> MLRRALLCLAVAALVRADAPEEEDHVLVLRKSNFAEALAAHKYLLVEFYAPWCGHCKALAPEYAKAAGKLKAEGSEIRLAKVDATEESDLAQQYGVRGYPTIKFFRNGDTASPKEYTAGREADDIVNWLKKRTGPAATTLPDGAAAESLVESSEVAVIGFFKDVESDSAKQFLQAAEAIDDIPFGITSNSDVFSKYQLDKDGVVLFKKFDEGRNNFEGEVTKENLLDFIKHNQLPLVIEFTEQTAPKIFGGEIKTHILLFLPKSVSDYDGKLSNFKTAAESFKGKILFIFIDSDHTDNQRILEFFGLKKEECPAVRLITLEEEMTKYKPESEELTAERITEFCHRFLEGKIKPHLMSQELPEDWDKQPVKVLVGKNFEDVAFDEKKNVFVEFYAPWCGHCKQLAPIWDKLGETYKDHENIVIAKMDSTANEVEAVKVHSFPTLKFFPASADRTVIDYNGERTLDGFKKFLESGGQDGAGDDDDLEDLEEAEEPDMEEDDDQKAVKDEL;> MILLAVLFLCFISSYSASVKGHTTGLSLNNDRLYKLTYSTEVLLDRGKGKLQDSVGYRISSNVDVALLWRNPDGDDDQLIQITMKDVNVENVNQQRGEKSIFKGKSPSKIMGKENLEALQRPTLLHLIHGKVKEFYSYQNEAVAIENIKRGLASLFQTQLSSGTTNEVDISGNCKVTYQAHQDKVIKIKALDSCKIARSGFTTPNQVLGVSSKATSVTTYKIEDSFVIAVLAEETHNFGLNFLQTIKGKIVSKQKLELKTTEAGPRLMSGKQAAAIIKAVDSKYTAIPIVGQVFQSHCKGCPSLSELWRSTRKYLQPDNLSKAEAVRNFLAFIQHLRTAKKEEILQILKMENKEVLPQLVDAVTSAQTSDSLEAILDFLDFKSDSSIILQERFLYACGFASHPNEELLRALISKFKGSIGSSDIRETVMIIT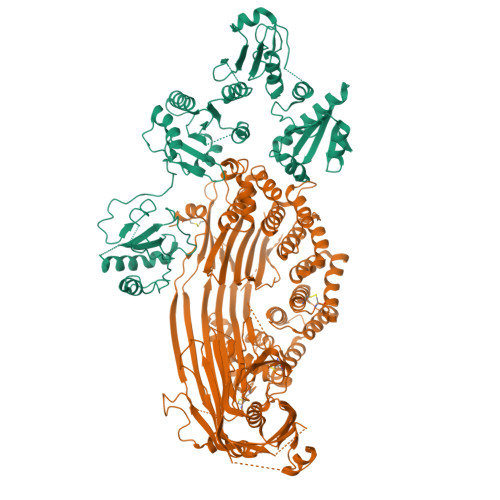GTLVRKLCQNEGCKLKAVVEAKKLILGGLEKAEKKEDTRMYLLALKNALLPEGIPSLLKYAEAGEGPISHLATTALQRYDLPFITDEVKKTLNRIYHQNRKVHEKTVRTAAAAIILNNNPSYMDVKNILLSIGELPQEMNKYMLAIVQDILRFEMPASKIVRRVLKEMVAHNYDRFSRSGSSSAYTGYIERSPRSASTYSLDILYSGSGILRRSNLNIFQYIGKAGLHGSQVVIEAQGLEALIAATPDEGEENLDSYAGMSAILFDVQLRPVTFFNGYSDLMSKMLSASGDPISVVKGLILLIDHSQELQLQSGLKANIEVQGGLAIDISGAMEFSLWYRESKTRVKNRVTVVITTDITVDSSFVKAGLETSTETEAGLEFISTVQFSQYPFLVCMQMDKDEAPFRQFEKKYERLSTGRGYVSQKRKESVLAGCEFPLHQENSEMCKVVFAPQPDSTSSGWF> MSATKSIVGEALEYVNIGLSHFLALPLAQRISLIIIIPFIYNIVWQLLYSLRKDRPPLVFYWIPWVGSAVVYGMKPYEFFEECQKKYGDIFSFVLLGRVMTVYLGPKGHEFVFNAKLADVSAEAAYAHLTTPVFGKGVIHDCPNSRLMEQKKFVKGALTKEAFKSYVPLIAEEVYKYFRDSKNFRLNERTTGTIDVMVTQPEMTIFTASRSLLGKEMRAKLDTDFAYLYSDLDKGFTPINFVFPNLPLEHYRKRDHAQKAISGTYMSLIKERRKNNDIQDRDLIDSLMKNSTYKDGVKMTDQEIANLLIGVLMGGQHTSAATSAWILLHLAERPDVQQELYEEQMRVLDGG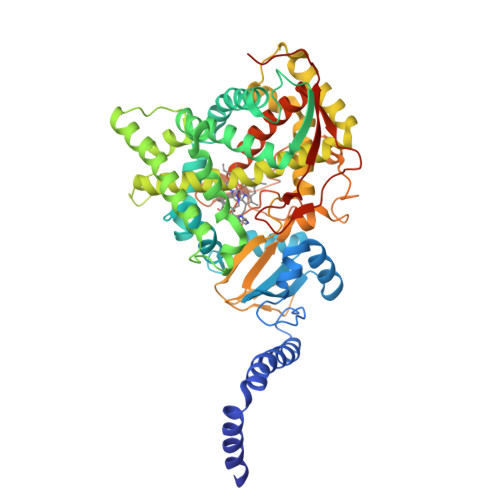KKELTYDLLQEMPLLNQTIKETLRMHHPLHSLFRKVMKDMHVPNTSYVIPAGYHVLVSPGYTHLRDEYFPNAHQFNIHRWNNDSASSYSVGEEVDYGFGAISKGVSSPYLPFGGGRHRCTGEHFAYCQLGVLMSIFIRTLKWHYPEGKTVPPPDFTSMVTLPTGPAKIIWEKRNPEQKIGGRHHHHHH(13Z)-docos-13-enamide | C22 H43 N O 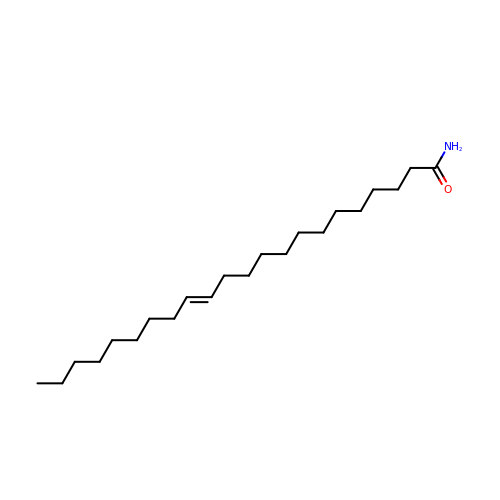| UAUDZVJPLUQNMU-KTKRTIGZSA-N>[8x]GHMSSMLPSISPELARIAPGFRALSINVIAAPIRD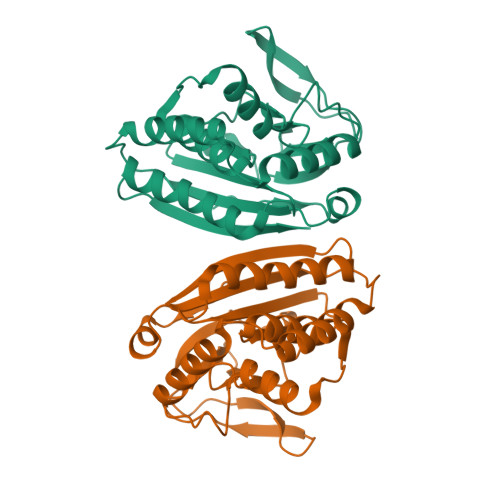AQVGEIALKEACQAVINGQPAWAQAHIDAWNTVLKAFGAKPKRTPCSAEALRKRVLKDGTMAALDPVVDLYNAVSLRYAVPVGGENSAAYCGSPRLVFADGSETFDTLKEGQPATESPEPGEVIWRDDRGVTCRRWNWRQGVRTRLSASDKAMWFILESLPEMPVDELYAAGNMLTDGLEKMMPGLRFESTLIGV> SQGASVLFGAPGAG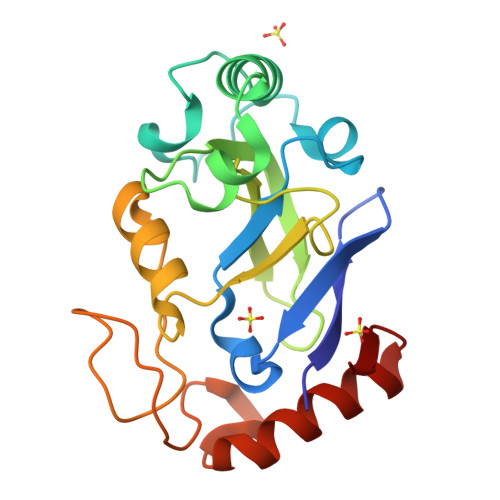DIEVFTTRPDTLFGATYMVLAPEHPLVDQLAADVWPQDTDPRWTGGQDSPRAAIEQYRRSIAAKSDLERQENKEKTGVFTGAYATNPVSGKPVPVFIADYVLLGYGTGAIMAVPGHDQRDWDFANTFGLPVQEVISGGDVTKAAYTGDGVLVNSDYLDGLDIEAAKVEVTRRLVKDGRGESR cyclopropane-1,1-dicarboxylic acid | C5 H6 O4 | 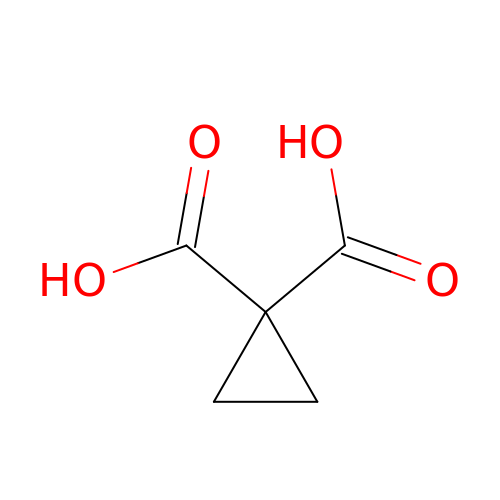FDKLLWKMYAMLIF-UHFFFAOYSA-N>MVMKLIGSHASPYTRKVRVVLAEKKIDYQFVLEDVWNADTQIHQFNPLGKVPCLVMDDGGALFDSRVIAEYADTLSPVARLIPPSGRERVEVRCWEALADGLLDAAVALRVEQTQRTPEQRSESWITRQHHKIDEALKAMSRGLADRTWCNGNHLTLADIAVGCALAYLDFRQPQVDWREQHANLAAFYTRIEKRPSFLETQPQAENLYFQS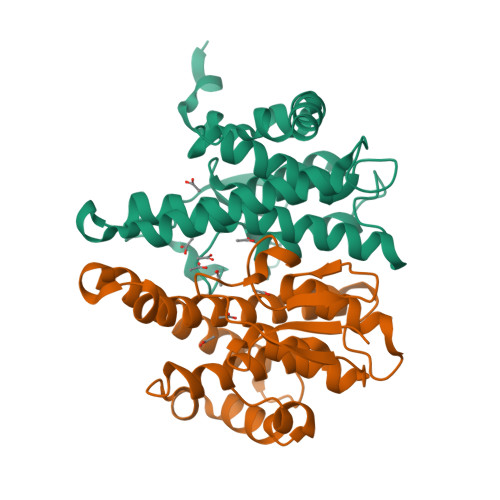HHHHHHWSHPQFEK[2x]>MIRYLRGLVLKKEAGGFVLLAGGVGFFLQAPTPFLQALEEGKEVGVHTHLLLKEEGLSLYGFPDEENLALFELLLSVSGVGPKVALALLSALPPRLLARALLEGDARLLTSASGVGRRLAERIALELKGKVPPHLLAGEKVESEAAEEAVMALAALGFKEAQARAVVLDLLAQNPKARAQDLIKEALKRLR[2x];> MEDLALRPKTLDEYIGQERLKQKLRVYLEAAKARKEPLEHLLLFGPPGLGKTTLAHVIAH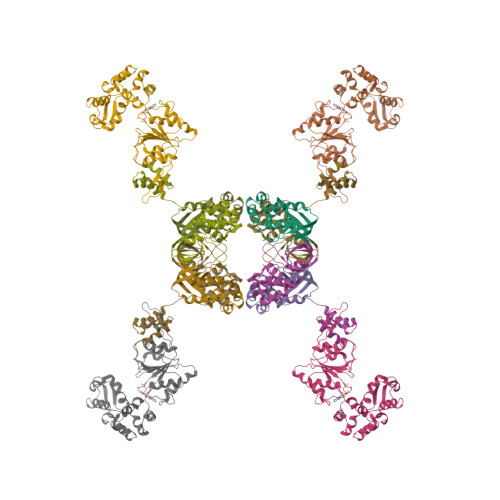ELGVNLRVTSGPAIEKPGDLAAILANSLEEGDILFIDEIHRLSRQAEEHLYPAMEDFVMDIVIGQGPAARTIRLELPRFTLIGATTRPGLITAPLLSRFGIVEHLEYYTPEELAQGVMRDARLLGVRITEEAALEIGRRSRGTMRVAKRLFRRVRDFAQVAGEEVITRERALEALAALGLDELGLEKRDREILEVLILRFGGGPVGLATLATALSEDPGTLEEVHEPYLIRQGLLKRTPRGRVATELARRHL>[2x]RSPWEGTLPAFLPCELQPHGQVDCNWLFLKSVPHFSAGAPRANVTSLSLISNRIHHLHDSDFVHLSNLRVLNLKWNCPPAGLSPMHFPCRMTIEPNTFLAVPTLEELNLSYNGITTVPALPSSLVSLSLSHTSILVLGPTHFTGLHALRFLYMDGNCYYMNPCPRALEVAPGALLGLGNLTHLSLKYNNLTEVPRRLPPSLDTLLLSYNHIVTLAPEDLANLTALRVLDVGGNCRR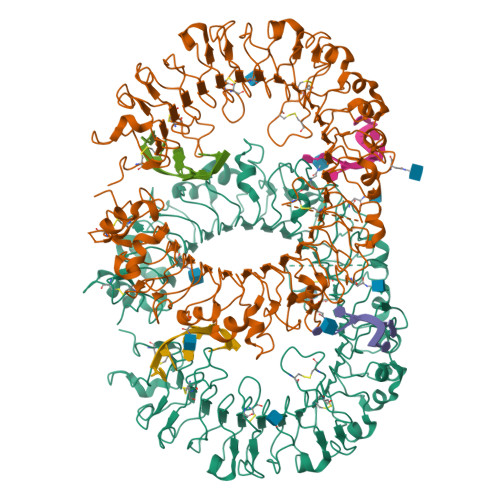CDHARNPCRECPKNFPKLHPDTFSHLSRLEGLVLKDSSLYKLEKDWFRGLGRLQVLDLSENFLYDYITKTTIFNDLTQLRRLNLSFNYHKKVSFAHLHLASSFGSLVSLEKLDMHGIFFRSLTNITLQSLTRLPKLQSLHLQLNFINQAQLSIFGAFPSLLFVDLSDNRISGAATPAAALGEVDSRVEVWRLPRGLAPGPLDAVSSKDFMPSCNLNFTLDLSRNNLVTIQQEMFTRLSRLQCLRLSHNSISQAVNGSQFVPLTSLRVLDLSHNKLDLYHGRSFTELPQLEALDLSYNSQPFSMQGVGHNLSFVAQLPSLRYLSLAHNGIHSRVSQKLSSASLRALDFSGNSLSQMWAEGDLYLCFFKGLRNLVQLDLSENHLHTLLPRHLDNLPKSLRQLRLRDNNLAFFNWSSLTVLPRLEALDLAGNQLKALSNGSLPPGIRLQKLDVSSNSIGFVIPGFFVRATRLIELNLSANALKTVDPSWFGSLAGTLKILDVSANPLHCACGAAFVDFLLERQEAVPGLSRRVTCGSPGQLQGRSIFTQDLRLCLDETLSLDEFLVPR> MSLEAIVFDRSEPENVSVKVLDQLLLPYTTKYVPIHTIDDGYSVIKSMQVRGAPAIAIVGSLSVLTEVQLIKHNPTSDVATLYSLVNWESTKTVLNKRLDFLLSSRPTAVNLSNSLVEIKNI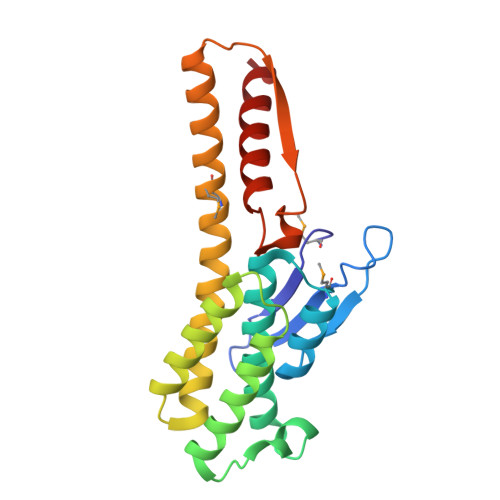LKSSSDLKAFDGSLYNYVCELIDEDLANNMKMGDNGAKYLIDVLQKDGFKDEFAVLTICNTGSLATSGYGTALGVIRSLWKDSLAKTDK> GPGSEVPTDGNAGLLAEPQIAMFCGKLNMHMNVQNGKWESDPSGTKTCIGTKEGILQYCQEVYPELQITNVVEANQPVTIQNWCKRGRKQCKTHTHIVIPYRCLVGEFVSDALLVPDKCKFLHQERM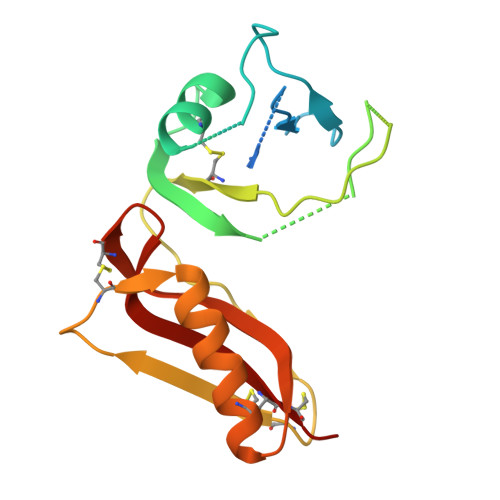DVCETHLHWHTVAKETCSEKSTNLHDYGMLLPCGIDKFRGVEFVCCPLA~{N}-[[1-(4-phenoxyphenyl)-1,2,3-triazol-4-yl]methyl]-2-(trifluoromethyl)pyridin-4-amine | C21 H16 F3 N5 O | 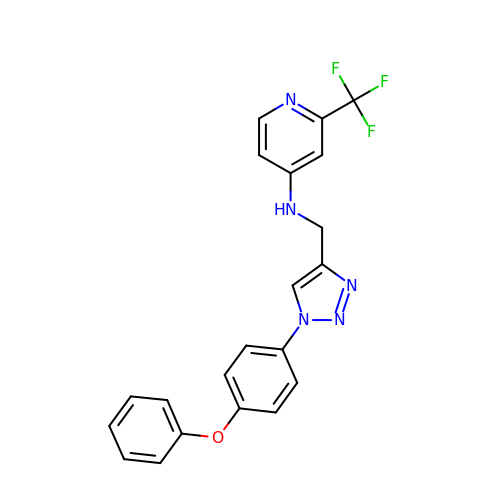QWSDRNYEGNKRGV-UHFFFAOYSA-N> AHHHHHHVDDDDKMQTVGVHSIVQQLHRNSIQFTDGYEVKEDIGVGSYSVCKRCIHKATNMEFAVKIIDKSKRDPTEEIEILLRYGQHPNIITLKDVYDDGKYVYVVMELMKGGELLDKILRQKFFSEREASAVLFTITKTVEYLHAQGVVHRDLKPSNILYVDESGNPESIRICDFGFAKQLRAENGLLMTPCYTANFVAPEVLERQGYDAACDIWSLGVLLYTMLTGYTPFANGPDDTPEEILARIGSGKFSLSGGYWNSVSDTAKDLVSKMLHVDPHQRLTA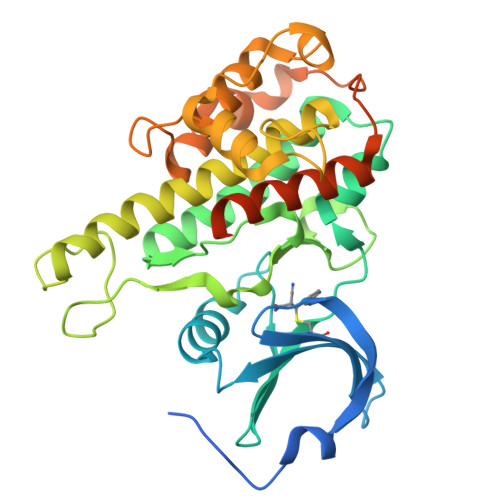ALVLRHPWIVHWDQLPQYQLNRQDAPHLVKGAMAATYSALNRNQSPVLEPVGRSTLAQRRGIKKITSTAL>[2x]HMSELSVATGAVSTASSSIPMPAGVNPADLAAELAAVVTESVDEDYLLYECDGQWVLAAGVQAMVELDSDELRVIRDGVTRRQQWSGRPGAALGEA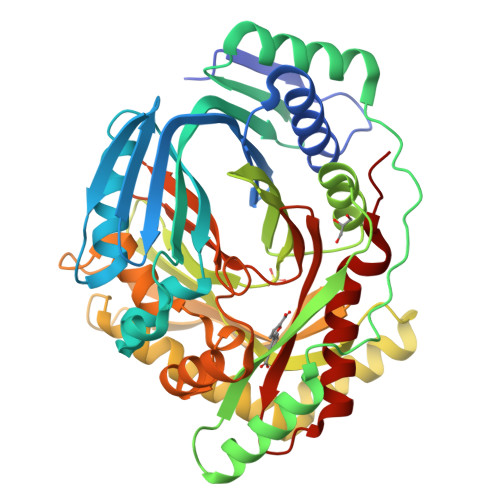VDRLLLETDQAFGWVAFEFGVHRYGLQQRLAPHTPLARVFSPRTRIMVSEKEIRLFDAGIRHREAIDRLLATGVREVPQSRSVDVSDDPSGFRRRVAVAVDEIAAGRYHKVILSRCVEVPFAIDFPLTYRLGRRHNTPVRSFLLQLGGIRALGYSPELVTAVRADGVVITEPLAGTRALGRGPAIDRLARDDLESNSKEIVEHAISVRSSLEEITDIAEPGSAAVIDFMTVRERGSVQHLGSTIRARLDPSSDRMAALEALFPAVTASGIPKAAGVEAIFRLDECPRGLYSGAVVMLSADGGLDAALTLRAAYQVGGRTWLRAGAGIIEESEPEREFEETCEKLSTLTPYLVARQ>MTGGMKPPARKPRILNSDGSSNITRLGLEKRGWLDDHYHDLLTVSWPVFITLITGLYLVTNALFA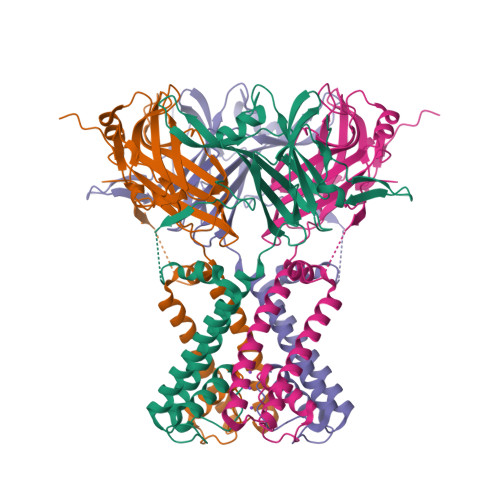LAYLACGDVIENARPGSFTDAFFFSVQTMATIGYGKLIPIGPLANTLVTLEALCGMLGLAVAASLIYARFTRPTAGVLFSSRMVISDFEGKPTLMMRLANLRIEQIIEADVHLVLVRSEISQEGMVFRRFHDLTLTRSRSPIFSLSWTVMHPIDHHSPIYGETDETLRNSHSEFLVLFTGHHEAFAQNVHARHAYSCDEIIWGGHFVDVFTTLPDGRRAIDLGKFHEIAQHHHHHH[8x]>GSGGIEGRHMVELLKLVRSSGCAAKVGPGDLQEILKGFNIYTDESTLVSIGDDAGVYEHNGIIWVYTVDIITPVVNDPYLWGAISTANALSDVYAMGGIPVNALAISCFNNCELDIEIFR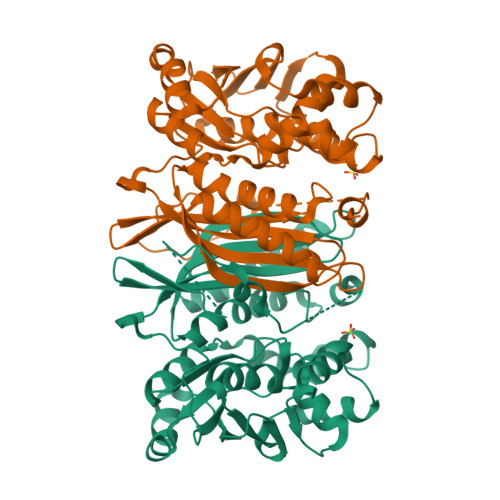EVIRGALDKLREAKTVLLGGHTIDDKEPKFGLSVAGICPEGKYITQSGAQVGQLLILTKPIGTGILIKGLKEGILKEEDINEAIENMLALNDKARNLMLSLDATACTDVTGFGLLGHAWNICKNSNIGARIFFEKVPYYQLSENLVKKKIYPKGAIENLNFVKNYLKSNLDNWKLILLSDPVTSGGLLFTINKEKLEKIDETAKELEVNYWIIGETIAENVLEVL[2x]>[2x]MSGQGFRSILTGSFSTPCADNPTVAMVEAGYHHAGLDARYINCDVKASGLADAVKGAKAMEWVGFNCSLPHKVAVLDHLDDIAESARLIGAVNCVAIREGKLIGHNTDGKGFLASLKTVTSPAGKRVVILGAGGAARAIAVELALAGAAHIT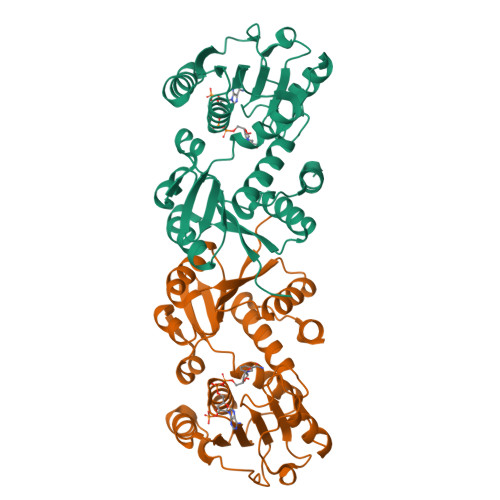IVNRDASKAETIAALINDKTEATGEAQAWSGKFSLPTGTDILINATSIGLGDPNAAPPVEMGSLTKETVVADVIPNPPQTRFLKDAKALGCTTLDGLGMLVNQGVIGVEIWLGRTLDSAVMAQTLENIFGTENK>[6x]MAPVIPSNTDYPGPHHFEVTFQQSSTAKSATWTYSPLLKKLYCQIAKTCPIQIKVSTPPPPGTAIRAMPVYKKAEHVTDVVKRCPNHELGRDFNEGQSAPASHLIRVEGNNLSQYVDDPVTGRQSVVVPYEPPQVGTEFTTILYNFMCNSSCVGGMNRRPILIIITLEMRDGQVLGRRSFEGRICACPGRDRKADEDHYREAENLYFQ;>[6x]SMPEITGQVSLPPGKRTNLRKTGSERIAHGMRVKFNPLALLLDSSLEGEFDLVQRIIYEVDDPSLPNDEGITALHNAVCAGHTEIVKFLVQFGVNVNAADSDGWTPLHCAASCNNVQVCKFLVESGAAVFAMTYSDMQTAADKCEEMEEGYTQCSQFLYGVQEKMGIMNKGVIYALWDYEPQNDDELPMKEGDCMTIIHREDEDEIEWWWARLNDKEGYVPRNLLGLYPRIKPRQRSLA

The p53 family of transcription factors comprises p53 and the paralogs p63 and p73.1 Under conditions of cellular stress, all three proteins are activated to induce genes necessary for cell cycle arrest or apoptosis. All three proteins share a similar domain organization containing an N-terminal transactivation domain, a DNA-binding domain (DBD) and a C-terminal oligomerization domain (OD).9 p63 and p73 contain an additional sterile α-motif domain and an inhibitory domain at the C-terminus. Both p63 and p73 share approximately 60% sequence identity with p53 in the DBD, and DNA contact residues are strictly conserved across all three proteins. To address the potential for similar p73 assembly, we solved the high‐resolution crystal structure of the DBD of p73 as well as its complex with the ankyrin repeat and SH3 domains of ASPP2.

Crystals of the complex were obtained in space group I121 when combining the p73 DBD with the ankyrin repeat and SH3 domains (residues 891–1128) of human ASPP2. The six p73 chains in the asymmetric unit were traceable between residues 114 and 311. Overall, the p73–ASPP2 structure is highly conserved with the p53 complex but exhibits a shift in the ASPP2 position to better accommodate the variant p73 L2 loop. As a result, the contact surface area of the p53–ASPP2 structure (753 Å2) is slightly greater than that of the p73–ASPP2 complex, which varies across the noncrystallographic‐symmetry‐related molecules from 672 to 742 Å2. The binding of both proteins is directed primarily by the L3 loop interaction with the ASPP2 SH3 domain but supported by further L2 loop contact with the fourth ankyrin repeat. The most significant contact is made by the cancer hotspot residue p53 R248 and the equivalent p73 residue R268, which was disordered in the unbound p73 structure. Both side chains undergo rearrangements to fill the large SH3 pocket formed between the RT and n-Src loops. Comparison of the two structures reveals that the n-Src loop in the p73 complex is moved ~ 6 Å away from its position in the equivalent p53 structure. To avoid a steric clash with p73 L199–R201, the fourth ankyrin repeat of ASPP2 is moved by ~2Å relative to the p53 complex and there is an ~180° change in the Ψ-angle of ASPP2 Y1023. Although the binding mode of p73 is similar to that of the p53–ASPP2 complex, we show that it requires additional structural rearrangements in ASPP2 to avoid steric clashes with the H1 helix, which bulges out from p73 due to its L2 loop insertion.> RSETTTSVRYHQSIRWKLVSEMKAENIKSFLRSFTKLPHLAGTEQNFLLAKKIQTQWKKFGLDSAKLVHYDVLLSYPNETNANYISIVDEHETEIFKTSYLEPPPDGYENVTNIVPPYNAFSAQGMPEGDLVYVNYARTEDFFKLEREMGINCTGKIVIARYGKIFRGNKVKNAMLAGAIGIILYSDPADYFAPEVQPYPKGWNLPGTAAQRGNVLNLNGAGDPLTPGYPAKEYTFRLDVEEGVGIPRIPVHPIGYNDAEILLRYLGGIAPPDKSWKGALNVSYSIGPGFTGSDSFRKVRMHVYNINKITRIYNVVGTIRGSVEPDRYVILGGHRDSWVFGAIDPTSGVAVLQEIARSFGKLMSKGWRPRRTIIFASWDAEEFGLLGSTEWAEENVKILQERSIAYINSDSSIEGNYTLRVDCTPLLYQLVYKLTKEIPSPDDGFESKSLYESWLEKDPSPENKNLPR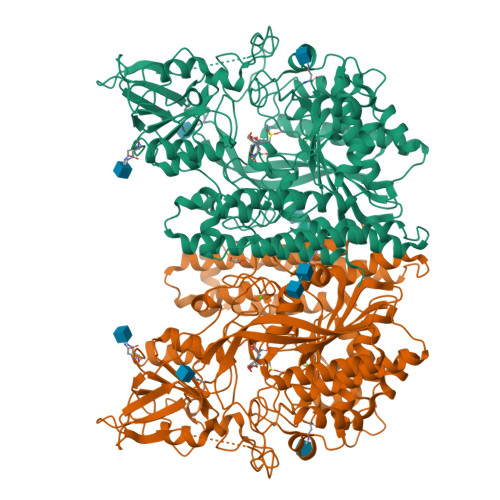INKLGSGSDFEAYFQRLGIASGRARYTKNKKTDKYSSYPVYHTIYETFELVEKFYDPTFKKQLSVAQLRGALVYELVDSKIIPFNIQDYAEALKNYAASIYNLSKKHDQQLTDHGVSFDSLFSAVKNFSEAASDFHKRLIQVDLNNPIAVRMMNDQLMLLERAFIDPLGLPGKLFYRHIIFAPSSHNKYAGESFPGIYDAIFDIENKANSRLAWKEVKKHISIAAFTIQAAAGTLKEVL Here we systematically compare RT fragment screening of the Fosfomycin-resistance protein A from Klebsiella pneumoniae (FosAKP), an enzyme involved in antibiotic resistance, with conventional single crystal data collection at cryogenic temperature (cryo). Fosfomycin, a broad-spectrum antibiotic, is routinely used to treat urinary infections. However, natural resistance can exist in gram-negative bacteria, mainly through the enzyme Fosfomycin-resistance protein A (FosA), that catalyzes the Mn2+ and K+-dependent glutathione mediated inactivation of Fosfomycin. Therefore, increased interest exists to identify inhibitors of FosA to enable the use of Fosfomycin to also treat resistant strains24.

For comparison, the same screen was conducted with conventional single crystal data collection at cryogenic temperatures (100 K) from loop-mounted crystals at beamline P11 at PETRA III. In total, 7 fragments bind in the two RT screens, of which 3 bind to pharmaceutically relevant sites 1, 2 and 4. In contrast, 31 fragments are observed binding in the cryo screens, but only 6 of these bind to the more interesting sites 1-4.

>[2x]MLSGLNHLTLAVSQLAPSVAFYQQLLGMTLHARWDSGAYLSCGDLWLCLSLDPQRRVTPPEESDYTHYAFSISEADFASFAARLEAAGVAVWKLNRSEGASHYFLDPDGHKLELHVGSLAQRLAACREQPYKGMVFFEQHHHHHH>MNKTYAACPQNWIGVENKCFYFSEYPSNWTFAQAFCMAQEAQLARFDN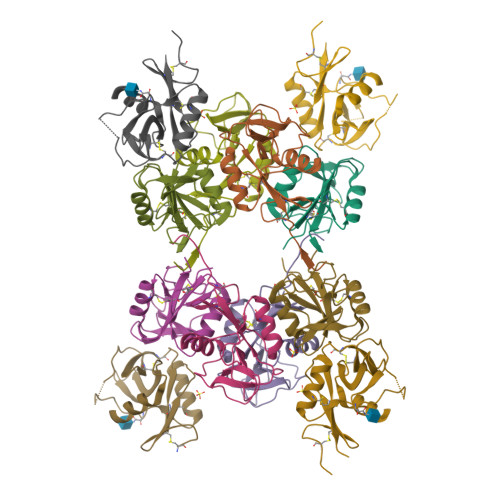QDELNFLMRYKANFDSWIGLHRESSEHPWKWTDNTEYNNTIPIRGEERFAYLNNNGISSTRIYSLRMWICSKLNAS[16x];>TGSAKLECPQDWLSHRDKCFHVSQVSNTWKEGRIDCDKKGATLLLIQDQEELRFLLDSIKEKYNSFWIGLSYTLTDMNWKWINGTAFNSDVLKITGVTENGSCAAISGEKVTSEGCSSDNRWICQKELNGTHHHHHH[8x]> IVRPVADFSPSLWGDQFLSFSIKNQVAEKYAKEIEALKEQTRNMLLATGMKLADTLNLIDTIERLGISYHFEK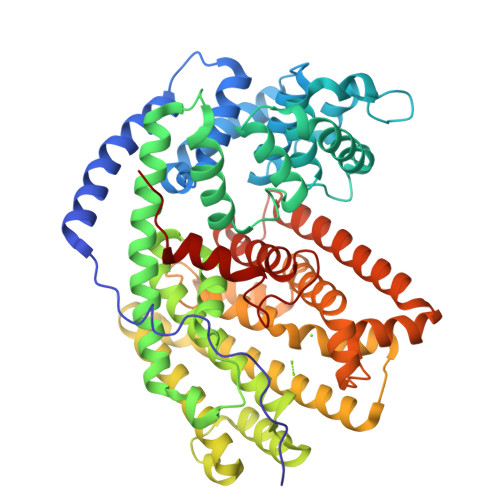EIDDILDQIYNQNSNCNDLCTSALQFRLLRQHGFNISPEIFSKFQDENGKFKESLASDVLGLLNLYEASHVRTHADDILEDALAFSTIHLESAAPHLKSPLREQVTHALEQCLHKGVPRVETRFFISSIYDKEQSKNNVLLRFAKLDFNLLQMLHKQELAQVSRWWKDLDFVTTLPYARDRVVECYFEALGVYFEPQYSQARVMLVKTISMISIVDDTFDAYGTVKELEAYTDAIQRWDINEIDRLPDYMKISYKAILDLYKDYEKELSSAGRSHIVCHAIERMKEVVRNYNVESTWFIEGYTPPVSEYLSNALATTTYYYLATTSYLGMKSATEQDFEWLSKNPKILEASVIICRVIDDTATYEVEKSRGQIATGIECCMRDYGISTKEAMAKFQNMAETAWKDINEGLLRPTPVSTEFLTPILNLARIVEVTYIHNLDGYTHPEKVLKPHIINLLVDSIKI>AVQVTFTVQKGSDPKKLVLDIKYTRPGDSLAEVELRQHGSEEWEPLTKKGNVWEVKSSKPLVGPFNFRFMSKGGMRNVFDEVIPTA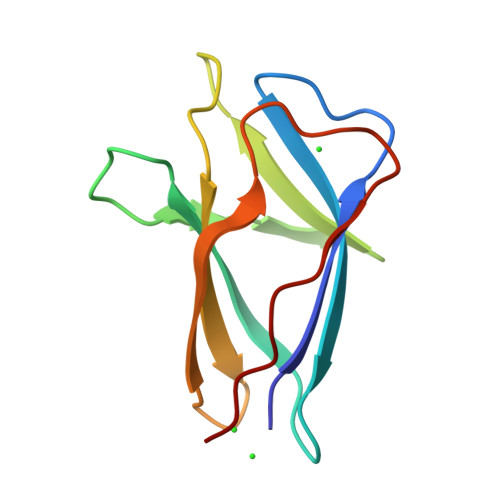FSIGKTYKPEEQEF[4x]>[4x]MRIPLVGKDSIESKDIGFTLIHEHLRVFSEAVRQQWPHLYNEDEEFRNAVNEVKRAMQFGVKTIVDPTVMGLGRDIRFMEKVVKATGINLVAGTGIYIYIDLPFYFLNRSIDEIADLFIHDIKEGIQGTLNKAGFVKIAADEPGITKDVEKVIRAAAIANKETKVPIITHSNAHNNTGLEQQRILTEEGVDPGKILIGHLGDTDNIDYIKKIADKGSFIGLDRYGLDLFLPVDKRNETTLRLIKDGYSDKIMISHDYCCTIDMGTAKPEYKPKLAPRWSITLIFEDTIPFLKRNGVNEEVIATIFKENPKKFFS

PLLs are natural lactonases endowed with promiscuous phosphotriesterase activity. The catalytic center contained two metal cations coordinated by four histidines, an aspartic acid and a carboxylated lysine residue. A structural analysis of SsoPox, a hyperthermostable counterpart of the PLL family from Sulfolobus solfataricus, has revealed that loop 7 is shorter in SsoPox than in PTEs; linking the active site to the loop 8, which forms a hydrophobic channel that accommodates AHLs aliphatic chain. Indeed, W263 is located at the start of loop 8, involved in the dimer interface of the enzyme and positions the lactone cycle of the substrate onto the bi-metallic catalytic center.

Compared to wild-type SsoPox, variants W263L, W263M and W263F are the most efficient at improving specific activities, ranging from 30-50 and 20-35-fold at 1 mM and 100 µM, respectively. These variants constitute the Phosphotriesterase Selected Variants group (PteSV). Variant W263F is the most proficient (kcat/KM = 1.21 (±0.26)x104 M-1s-1), followed by W263M and W263L with increased efficiencies of 23.3, 14.1 and 4.6-fold, respectively, as compared to wild-type enzyme. Regarding the PteSV group, while these variants exhibit higher phosphotriesterase activity, they demonstrate mild improvements for the oxo-lactones and no or wild-type-like AHLase activity (W263L-M and W263F, respectively). Notably, contrary to the wild-type enzyme, all selected variants (with the exception of W263F) exhibit a substrate inhibition for undecanoic-δ-lactones with KI values ranging between 789 ± 186 µM and 7 400 ± 2 475 µM, respectively, for the W263V and W263M variants. The analysis of the normalized B-factors of the variants clearly reveal that the substitution W263 is destabilizing (as confirmed by the Tm of the variants), but also that the active site loops of PteSV are significantly more disordered than those of LacSV. PteSV lose their activity before the loss of the global structure (Tm), whereas LacSV do not, and exhibit a similar thermophilicity profile to that of the wild-type enzyme. These data strongly suggest that the increased disorder in loop 8 caused by the PteSV substitutions collapses the loop as the temperature increase, whereas it does not occur with the LacSV.> SMQEEDTFRELRIFLRNVTHRLAIDKRFRVFTKPVDPDEVPDYVTVIKQPMDLSSVISKIDLHKYLTVKDYLRDIDLICSNALEAAPDRDP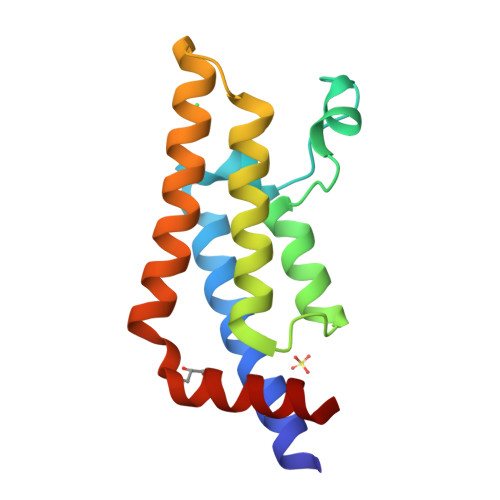GDRLIRHRACALRDTAYAIIKEELDEDFEQLCEEIQESR> GSSGSSGNWIDVRYDLE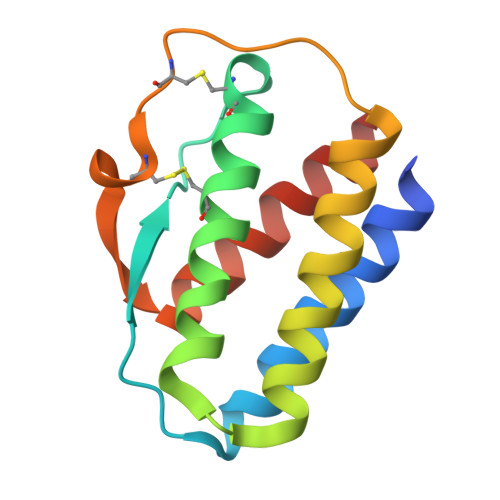KIESLIQSIHIDTTLYTDSDFHPSCKVTAMNCFLLELQVILHEYSNMTLNETVRNVLYLANSTLSSNKNVAESGCKECEELEEKTFTEFLQSFIRIVQMFINTS> GSHMGSPNSPLKDSLRPKLSEEQQHIIAI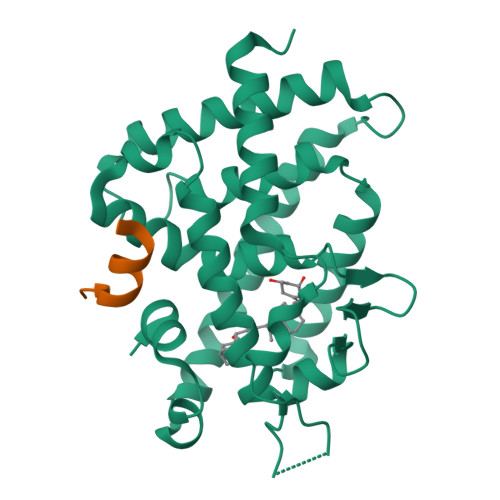LLDAHHKTYDPTYADFRDFRPPVRMDGSTGSVTLDLSPLSMLPHLADLVSYSIQKVIGFAKMIPGFRDLTSDDQIVLLKSSAIEVIMLRSNQSFTMDDMSWDCGSQDYKYDVTDVSKAGHTLELIEPLIKFQVGLKKLNLHEEEHVLLMAICIVSPDRPGVQDAKLVEAIQDRLSNTLQTYIRCRHPPPGSHQLYAKMIQKLADLRSLNEEHSKQYRSLSFQPENSMKLTPLVLEVFGNEIS;> KNHPMLMNLLKDN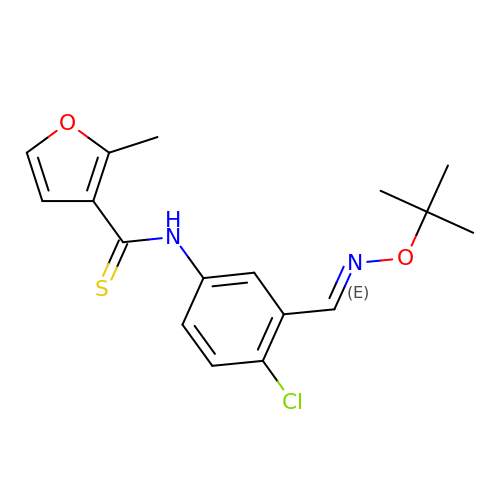N-[4-CLORO-3-(T-BUTYLOXOME)PHENYL-2-METHYL-3-FURAN-CARBOTHIAMIDE | C17 H19 Cl N2 O2 S | PLGIIOKXCKDKEU-VXLYETTFSA-N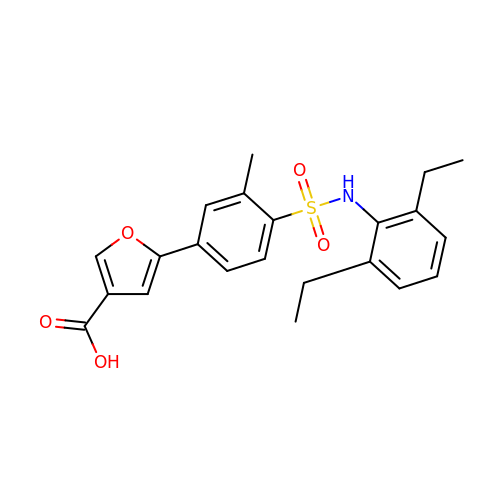5-[4-[(2,6-diethylphenyl)sulfamoyl]-3-methyl-phenyl]furan-3-carboxylic acid | C22 H23 N O5 S | SECRWZHINJOGSU-UHFFFAOYSA-N> GAGCAGCCCGTACTCG;> TC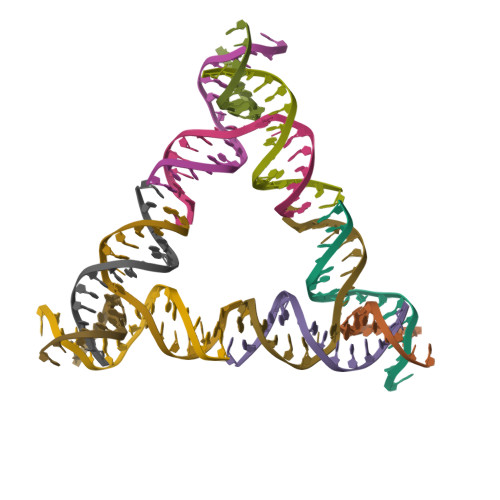TGATGAGGCTGC;> GCTTGTCGTTCATCA;> CCGAGTACGACGACAAG>SVSIQAFTLEYIEVATERYKTLIGEGGFGSVYRGTLNDGQEVAVKVRS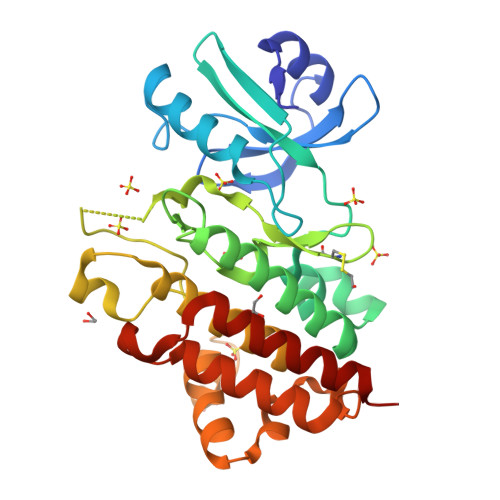ATSTQGTREFDNELNLLSAIQHENLVPLLGYCNESDQQILVYPFMSNGSLQDRLYGEPAKRKILDWPTRLSIALGAARGLAYLHTFPGRSVIHRDIKSSNILLDHSMCAKVANFGFSKYAPQEGDSYVSLEVRGTAGYLDPEYYKTQQLSEKSDVFSFGVVLLEIVSGREPLNIKRPRTEWSLVEWATPYIRGSKVDEIVDPGIKGGYHAEAMWRVVEVALQCLEPFSTYRPSMVAIVRELEDALIIENNAS[3x]> MVESDSSGIVRHSQGEFDIVQVYKKFLQDDPEITMPVAAIEALVQLLSRSQAKTISEFMDILQNGSNTLKEGVQNNISLSAGCDIFQRFVTRSLHDVGDFEQCKRHLVENGKLFIQRARACRQRIAHLGYPLIRDGSVILTHGFSRGVAAVLLAAAKRHVRFKVFVTES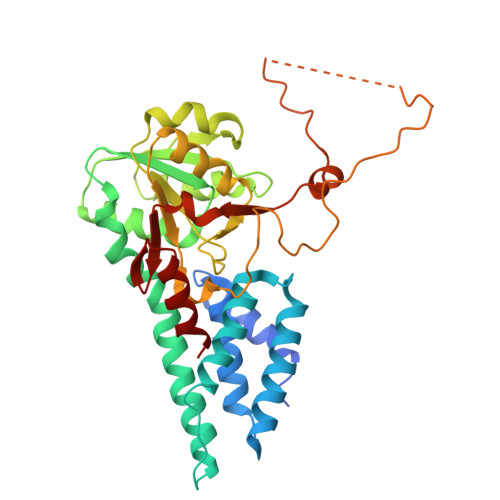RPSGSGCLMTRTLKNACIPTCMVLDSAVSFTMNRVDLVLVGAEGVVENGGLINQIGTFQLAVFAKHAHKPFYAVAESHKFVRMFPLSQYDIPFSRPILEFDDPSPETVHPEPEPIPTPSDAIHNELIMNEEQIRNNPTLDVTPPEFVSGLITDLGIIDSKSGVSEELIKLYL4-(3-hydroxyphenoxy)benzoic 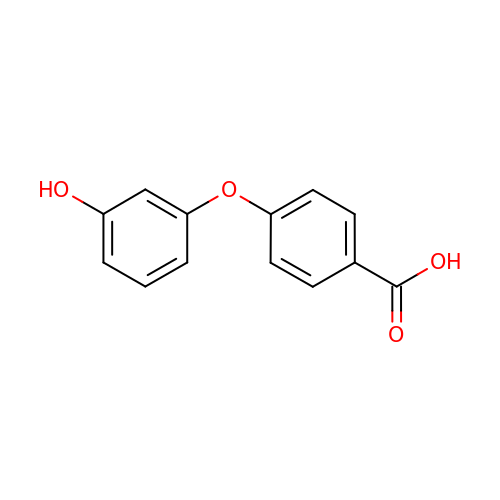acid | C13 H10 O4 | DEDKCEDXZJIDKZ-UHFFFAOYSA-N> EEPSSNEIHIGSLVIFPDAYVVSKRDETIELTHREFELLHYLAKHIGQVMTREHLLQTVWGYDYFGDVRTVDVTVRRLREKIEDNPSHPNWIVTRRGVGYY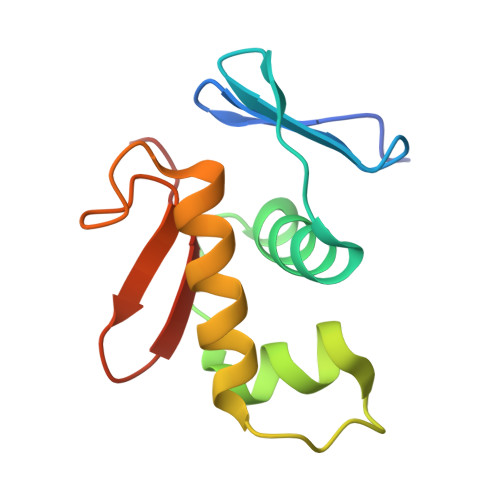LRNPEQD>[2x]MPASLLRFLALAGTAVGLTTNHNHSPSCRVLPGDAAWPSSRDWAKLNKTLNGHLIATVPQASVCHKSPFGQYDAQACEELKSSWDISTITHVNAPGDVLSQNFQNYSCVPFTDPSQPCQLGNYPSYVVNVTGAADVQAALKFAQKHNVRIVIKNTGHDYLGKSTGKGALSLWMHNLKSTKFIK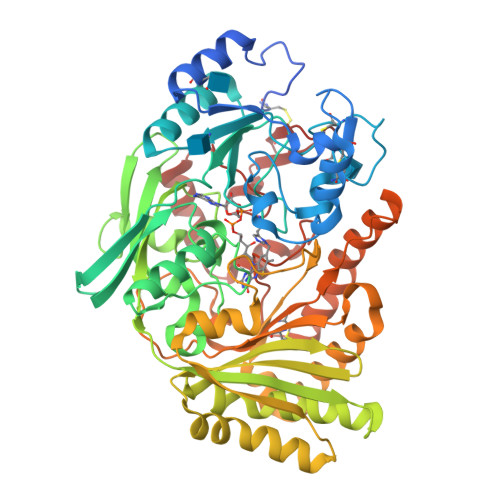NYKAPYYKGPAAKLGAGVEGFEAYAMANSTGHRIVGGTCPTVGIVGGYTQGGGHSILSSSYGVAADNVLEWEVVTADGRHLVATPTRNSDLYWALSGGGGGTFAVVLSMTARLHRDGIVGGTLLGFNDSAVGNEVYWEAVAAFHALLPDFLDGGNSFTYSVGNNSLTAYGTMPGADRDAVDRLLRPFLDDLASRGITPVVQPRVSTNYYDHFFTYLGPAPYGNAAYFPFTNSRIIPRSLVTDPKSNAVVTDLFRNISQVPAFSPFYCDSFSVADKPHPANSLHPAWRTGMLLCAPAGSWDWDASPEEMAARDRYAAETLQPMMDAATPGGSVYLNEANHLYANWKESFYGDNYARLLRVKKKYDPDSVFYVKTGVGSEVWDVDATGRLCRA3-(2-phenylimidazo[1,2-a]pyridin-6-yl)benzenecarbonitrile | C20 H13 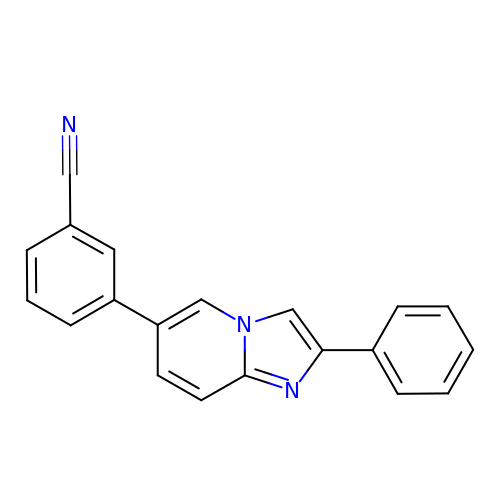N3 | ZIPMVBBAKJZVIG-UHFFFAOYSA-N>MAYRIVSETGDKITVELTLANKNTHYVWNGWCFDIKNITFETTGKVLSIKYADGGEPVYNVNGNLVTIDLTWRGIFHLNTTVKIIIEIQKSGDNPYPHNFKIHYLRGESIIYPTIGELPASWKPGNFTLSDLIADPKSYYDPHVKPHQNGFIMYNPPHPTQIIIGLADIDYPLNLASSARMWVPNKYFAMGLALAYEWFKVNPNFLMALAAKENWGTAVTKDPAFKGYKVIIDEEEYYWPVQIDHPDGIFQVESGNFNQIKAYYPDIFPDTADHDDYMKVSLDPNDTAWITSPIVAAVSLTMERELLYAAVGDKYNEFLRLAKDPWAETEIIDFGYNRGVGAIEALKIFSDNWEKAINAEVLWKEFNMEGFGGHVPTVINITATMDMETERIYDANLTWDDIEYFFTVVRQKFFRPGAISDEEWNAMMRDVKRAYDLLSQHWGGDHISYRY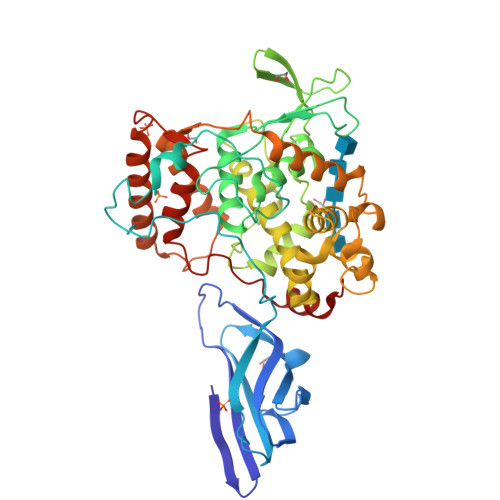DFLTILRVAMKHWPEPHIPRPTGDDWYYHARNYNP[2x]>[6x]MALRFITAEEAAEFVHHNDNVGFSGFTPAGNPK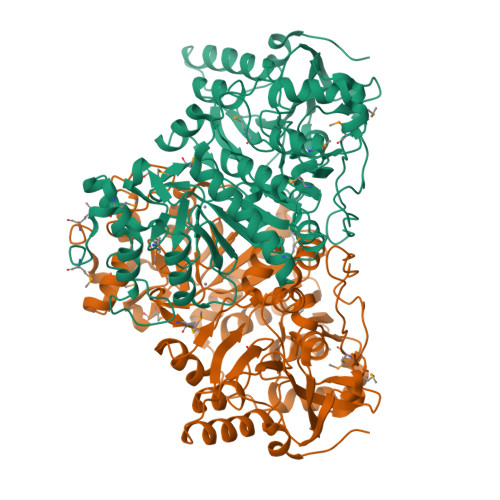VVPAAIAKRAIAAHEKGNPFKIGMFTGASTGARLDGVLAQADAVKFRTPYQSNKDLRNLINNGSTSYFDLHLSTLAQDLRYGFYGKVDVAIIEVADVTEDGKILPTTGVGILPTICRLADRIIVELNDKHPKEIMGMHDLCEPLDPPARRELPVYTPSDRIGKPYVQVDPAKIVGVVRTSEPNDESDFAPLDPVTQAIGDNVAAFLVSEMKAGRIPKDFLPLQSGVGNVANAVLGALGDNPDIPAFNMYTEVIQDAVIALMKKGRIKFASGCSLSVSRSVIQDIYANLDFFKDKILLRPQEYSNNPEIVRRLGVITINTALEADIFGNINSTHVSGTRMMNGIGGSGDFTRNSYVSIFTTPSVMKDGKISSFVPMVAHHDHSEHSVKVIISEWGVADLRGKNPRERAHEIIDKCVHPDYRPLLRQYLELGVKGQTPQNLDCCFAFHQELAKSGDMRNVRWEDYMKLEHHHHHH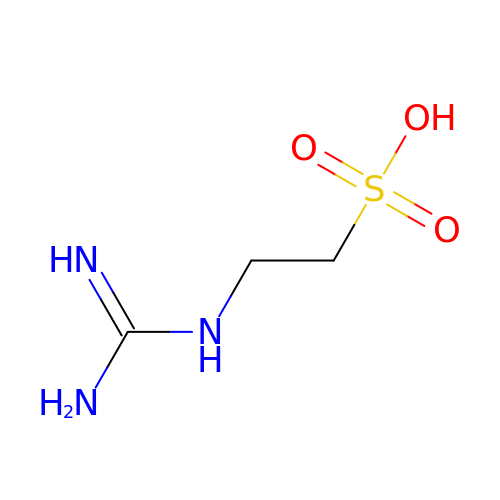Taurocyamine | C3 H9 N3 O3 S | JKLRIMRKZBSSED-UHFFFAOYSA-N>MHGEQWNTTAKVRPKNGPPYRVLQANLQRKKLATAELAIEAATRKAAIALIQEPYVGGAKSMKGFRGVRVFQSTAQGDGTVKAAIAVFDHDLDVIQYPQLTTNNIVVVGIRTRAWEITLVSYYFEPD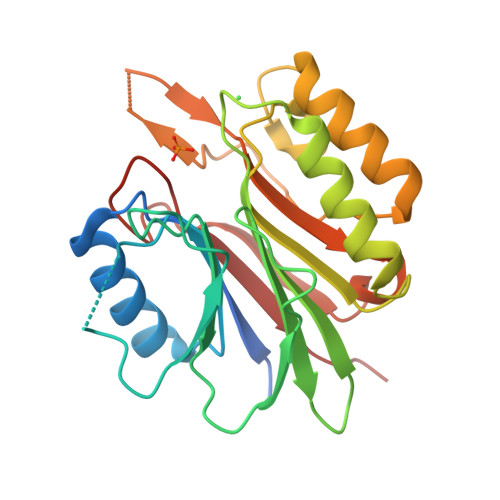KPIESYLEQIKRVERKMGPKRLIFGGDANAKSTWWGSKEDDARGDQLMGTLGELGLHILNEGDVPTFDTIRGGKRYQSRVDVTFCTEDMLDLIDGWRVDEDLVSSDHNGMVFNIRLQK[2x]> GSHMDGTEKWRFKTNDAITSAASIGKDGTIYFGSDKVYAINPDGTEKWNFYAGYWTVTRPAISEDGTIYVTSLDGHLYAINPDGTEKWRFKTEKRIESSPVIGNTDTIYFGSYDGHLYAINPDGTEKWRFKTNDAITSAAS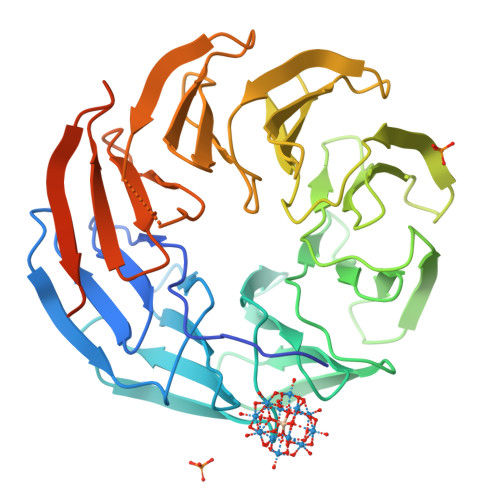IGKDGTIYFGSDKVYAINPDGTEKWNFYAGYWTVTRPAISEDGTIYVTSLDGHLYAINPDGTEKWRFKTEKRIESSPVIGNTDTIYFGSYDGHLYAINPDGTEKWRFKTNDAITSAASIGKDGTIYFGSDKVYAINPDGTEKWNFYAGYWTVTRPAISEDGTIYVTSLDGHLYAINPDGTEKWRFKTEKRIESSPVIGNTDTIYFGSYDGHLYAINP> MLSVQKEFHGTIDYGDVTVTGGISVFDAKFDELYVYDGDDLGAVYAPEETRFRLWAPTASEAFVVLYETEDGMPVKELPMKRDVQGTWTLTVAEDCGGLFYTYRVKVGEQWNEAVDPYAKAVGVNGTKTAILDLRSTNPEGWENDQKPPLASPTDAVIYELHVRDLSIHPQSGIREKGKFLGLTEEGTRGPNGIPTGLDHITGLGVTHVQLLPIYDYSQESVDESRLDEPHYNWGYDPQNYNVPEGSYSTDPHNPAARILELKRLIQKLHARGLRVIMDVVYNHVYDGYLIHFTKLVPGYYLRYKADRTFSDGTFCGNECASERPIMRKYIIESILHWVREYHIDGFRFALMGMIDIETMNEIRRRLDEIDPTILTIGEGWMMETVLPKELRANQDNAEKLPGIGMFNDGMRDAVKGDIFIFDRKGFISGGDGFEDGVKRGVAGGINYGGQLRQFAVEPVQSVNYVECHDNHTLWDKIELSTPGASDEER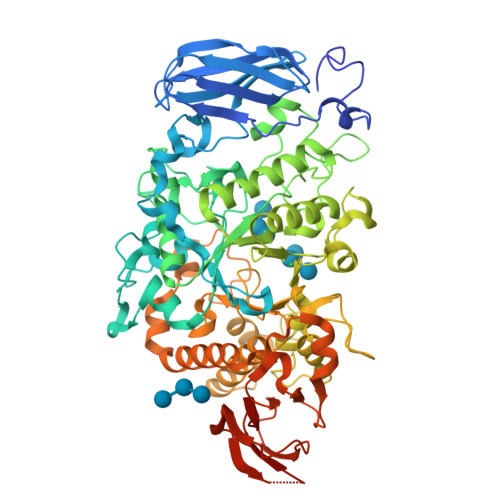RAMHRLASAIVLTSQGIPFLHAGQEFMRTKGGVENSYKSPIEVNWLDWERCAAHQDDVSYMRSLIALRKAHPAFRLKTADEIRAHLRFEAAPPHTVAFTLRDHAGGDPDRHLYVLYNANPGALSLELPALGPWEVRFGGEHVLALEAGASGEAAAAAPAAAGGPPAGGARLEVRGVGVVVLAVPR>[2x]VALSAEGSSGGSRGGSPKAEAASVPSWPQILGRLTDNRDLARGQAAWAMDQIMTGNARPAQIAAFAVAMTMKAPTADEVGELAGVMLSHAHPLPADTVPDDAVDVVGTGGDGVNTVNLSTMAAIVVAAAGVPVVKHGNRAASSLSG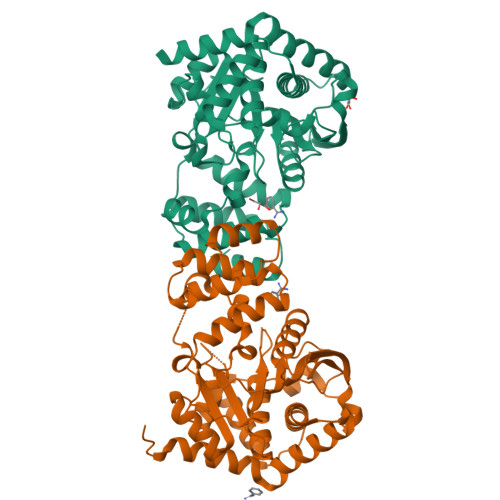GADTLEALGVRIDLGPDLVARSLAEVGIGFCFAPRFHPSYRHAAAVRREIGVPTVFNLLGPLTNPARPRAGLIGCAFADLAEVMAGVFAARRSSVLVVHGDDGLDELTTTTTSTIWRVAAGSVDKLTFDPAGFGFARAQLDQLAGGDAQANAAAVRAVLGGARGPVRDAVVLNAAGAIVAHAGLSSRAEWLPAWEEGLRRASAAIDTGAAEQLLARWVRFGRQILAA>[2x]MGFLSGKRILVTGVASKLSIAYGIAQAMHREGAELAFTYQNDKLKGRVEEFAAQLGSDIVLQCDV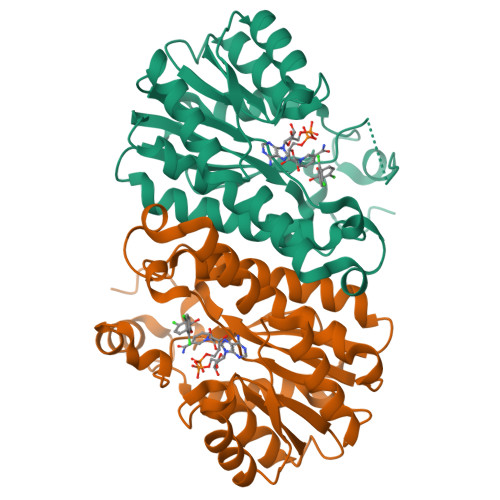AEDASIDTMFAELGKVWPKFDGFVHSIVFAPGDQLDGDYVNAVTREGFKIAHDISSYSFVAMAKACRSMLNPGSALLTLSYLGAERAIPNYNVMGLAKASLEANVRYMANAMGPEGVRVNAISAGPIRTLAASGIKDFRKMLAHCEAVTPIRRTVTIEDVGNSAAFLCSDLSAGISGEVVHVDGGFSIAAMNELELKLEHHHHHH> SDPTVFHKRYLKKIRDLGEGHFGKVSLYCYDPTNDGTGEMVAVKALKEGCGPQLRSGWQREIEILRTLYHE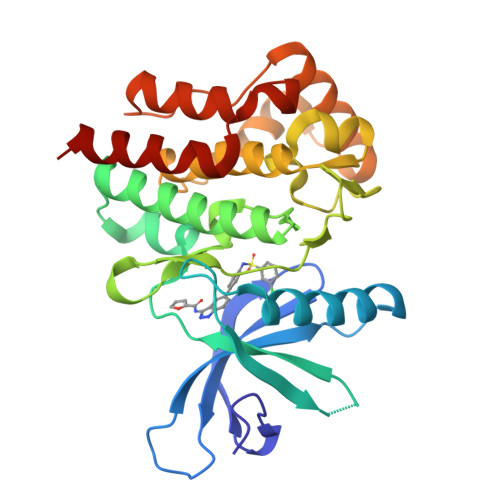HIVKYKGCCEDQGEKSVQLVMEYVPLGSLRDYLPRHCVGLAQLLLFAQQICEGMAYLHAQHYIHRALAARNVLLDNDRLVKIGDFGLAKAVPEGHEYYRVREDGDSPVFWYAPECLKECKFYYASDVWSFGVTLYELLTYCDSNQSPHTKFTELIGHTQGQMTVLRLTELLERGERLPRPDRCPCEIYHLMKNCWETEASFRPTFQNLVPILQTAQEKYQ> MKNTPQHKLFFVVALLLVVQILAGCKSSSSTTAGSTENSSSSTPDPDTGTTTPDPIEPEVVPPVTPPSVDSNSREVIPLWEDKVADGKAWSTHVYSALDKLGPNLLDVIPADRSLFCPKYSSLSY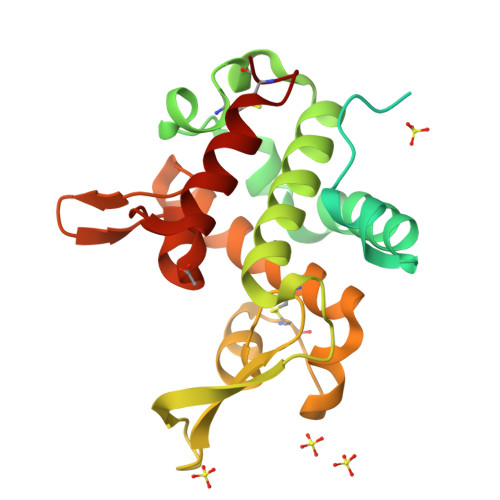AQRKQYWAFVLSSMVRFESNFKTAMSYTQDFNDSNGNRVISRGLLQISIESGNAYGCGFKSTKDLHDPLQNLSCGIRILDRWVSRDGRIAGKVDGAWKGGARYWSVLRAGDKTSYKSIVSWSQNLSICK>[12x]GNITDIKVSSLPNKQKIVKVSFDKEIVNPTGFVTSSPARIALDFEQTGISMDQQVLEYADPLLSKISAAQNSSRARLVLNLNKPGQYNTEVRGNKVWIFINESDDTVSAPARPAVKAAPAAPAKQQAAAPSTKSAVSVSEPFTPAKQQAAAPFTESVVSVSAPFSPAKQQAAASAKQQAAAPAKQQAAAPAKQQAAAPAKQTNIDFRKDGKNAGIIELAALGFAGQPDISQQHDHIIVTLKNHTLPTTLQRSLDVADFKTPVQKVTLKRLNNDTQLIITTAGNWELVNKSAAPGYFTFQVLPKKQNLESGGVNNAPKTFT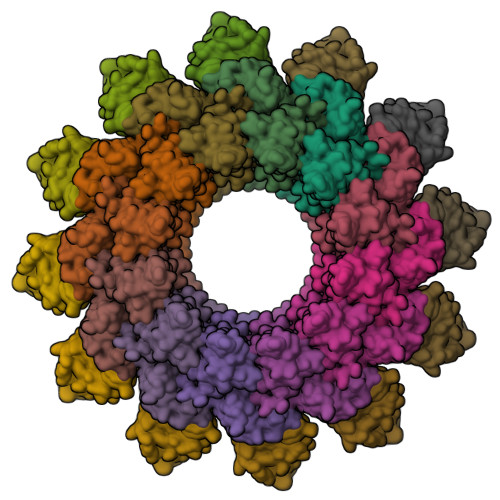GRKISLDFQDVEIRTILQILAKESGMNIVASDSVNGKMTLSLKDVPWDQALDLVMQARNLDMRQQGNIVNIAPRDELLAKDKAFLQAEKDIADLGALYSQNFQLKYKNVEEFRSILRLDNADTTGNRNTLISGRGSVLIDPATNTLIVTDTRSVIEKFRKLIDELDVPAQQVMIEARIVEAADGFSRDLGVKFGATGKKKLKNDTSAFGWGVNSGFGGDDKWGAETKINLPITAAANSISLVRAISSGALNLELSASESLSKTKTLANPRVLTQNRKEAKIESGYEIPFTVTSIANGGSSTNTELKKAVLGLTVTPNITPDGQIIMTVKINKDSPAQCASGNQTILCISTKNLNTQAMVENGGTLIVGGIYEEDNGNTLTKVPLLGDIPVIGNLFKTRGKKTDRRELLIFITPRIMGTAGNSLRY;>[12x]MKHYALLISFLALSACSQGSEDLNEWMAQTRREAKAEIIPFQAPTLPVAPVYSPPQLTGPNAFDFRRMETDKKGENAPDTKRIKETLEKFSLENMRYVGILKSGQKVSGFIEAEGYVYTVGVGNYLGQNYGRIESITDDSIVLNELIEDSTGNWVSRKAELLLNSSDKNTEQAAAPAAEQN> MGSSHHHHHHSSGRENLYFQGLSPQVRTAHIGDVPVLVRLMSEFYQEAGFALPHDAAIRAFKALLGKPDLGRIWLIAEGTESVGYIVLTLGFSMEYGGLRG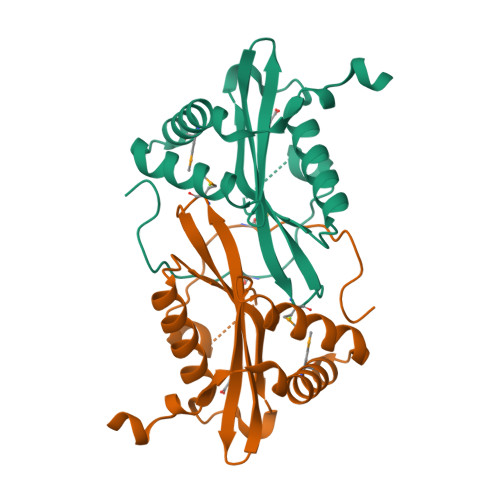FVDDFFVRPNARGKGLGAAALQTVKQGCCDLGVRALLVETGPEDHPARGVYSRAGFEESGRMLLGQALAPPIHEA>PLRMGGNGQLQYWPFSSSDLYNWKNNNPSFSEDPGKLTALIESVLTTHQPTWDDCQQLLGTLLTGEEKQRVLLEARKAVRGNDGRPTQLPNEVDAAFPLERPDWDYTTQRGRNHLVLYRQL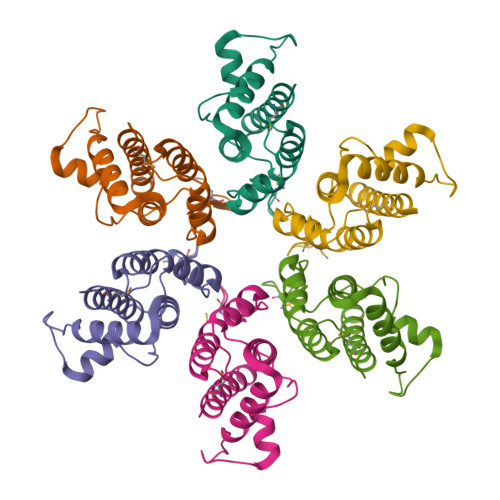LLAGMQNAGR[6x]> MASWSHPQFEKGSTSAFNPRDTVTVYFHAIVSRHFGFNPEEHKVYVRGGEGLGQKGWTDACEMYCTQDLHDLGSLVEGKMDIPRQSLDKPIPYKYVIHRGGSSKDTVEYEFIYEQAQKKGEHVNRCLRVVSTSLGNGDWHQYDDIICMRSTGFFQQAKNRILDSTRKELLKGKKQAAVVMLDRIFSVLQPWSDINLQSFMTQFLQFYSVVREPMIHDGRARKWTSLQYEEKEVWTNLWEHVKKQMAPFLEGKSGESLPADCPVRSKLTLGLSILFMVEAAEFTVPKKDLDSLCYLLIPSAGSPEALHSDLSPVLRIRQRWRIYLTNLCLRCIDERCDRWLGILPLLHTCMQKSPPKKNSKSQPEDTWAGLEGISFSEFRDKAPTRSQPLQFMQSKMALLRVDEYLFRSWLSVVPLESLSSYLENSIDYLSDVPVRVLDCLQGISYRLPGLRKISNQNMKKDVENVFKMLMHLVDIYQHRIFGENLLQIYLTECLTLHETVCNITANHQFFEIPALSAELICKLLELSPPGHTDEGLPEKSYEDLVTSTLQEALATTRNWLRSLFKSRMLSISSAYVRLTYSEEMAVWRRLVEIGFPEKHGWKGSLLGDMEGRLKQEPPRLQISFFCSSQCRDGGLHDSVSRSFEKCVIEAVSSACQSQTSVLEGLSCQDLQKFGTLLSAVITKSWPVHNGEPVFDVDEIFKYLLKWPDVRQLFELCGTNEKIIDNITEEGRQLMATAESVFQKVAGELENGTIVVGQLELILEHQSQFLDIWNLNRRRLPSQEKACDVRSLLKRRRDDLLFLKQEKRYVESLLRQLGRVKHLVQVDFGNIEIIHSQDLSNKKLNEAVIKLPNSSSYKRETHYCLSPDIREMASKLDSLKDSHIFQDFWQETAESLNTLDKDPRELKVSLPEVLEYLYNPCYDNFYTLYENLKSGKITFAEVDAIFKDFVDKYDELKNDLKFMCTMNPQDQKGWISERVGQIKEYHTLHQAVSSAKVILQVRRALGVTGDFSVLNPLLNFADSFEDFGNEKLDQISPQFIKAKQLLQDISEPRQRCLEELARQTELVAWLHKALEDINELKVFVDLASISAGENDIDVDRVACFHDAVQGYASLLYKMDERTNFSDFMNHLQELWRALDNDQHLPDKLKDSARNLEWLKTVKESHGSVELSSLSLATAINSRGVYVIEAPKDGQKISPDTVLRLLLPDGHGYPEALRTYSTEELKELLNKLMLMSGKKDHNSNTEVEKFSEVFSNMQRLVHVFIKLHCAGNMLFRTWTAKVYCCPDGGIFMNFGLELLSQLTEKGDVIQLLGALCRQMEDFLDNWKTVVAQKRAEHFYLNFYTAEQLVYLSSELRKPRPSEAALMMLSFIKGKCTVQDLVQATSACESKADRYCLREVMKKLPQQLLSEPSLMGKLQVIMMQSLVYMSAFLPHCLDLDALGRCLAHLATMGGTPVERPLPKGLQAGQPNLILCGHSEVLPAALAIYMQAPRQPLPTFDEVLLCTPATTIEEVELLLRRCLTSGSQGHKVYSLLFADQLSYEVGCQAEEFFQSLCTRAHREDYQLVILCDAAREHCYIPSTFSQYKVPLVPQAPLPNIQAYLQSHYQVPKRLLSAATVFRDGLCVGIVTSERAGVGKSLYVNTLHTKLKAKLRDETVPLKIIRLTEPHLDENQVLSALLPFLKEKYQKMPVIFHIDISTSVQTGIPIFLFKLLILQYLMDINGKIWRRSPGHLYLVEIPQGLSVQPKRSSKLNARAPLFKFLDLFPKVTCRPPKEVIDMELTPERSHTDPAMDPVEFCSEAFQRPYQYLKRFHQQQNLDTFQYEKGSVEGSPEECLQHFLIYCGLINPSWSELRNFAWFLNCQLKDCEASIFCKSAFTGDTLRGFKNFVVTFMILMARDFATPTLHTSDQSPGRQSVTIGEVVEEDLAPFSLRKRWESEPHPYVFFNGDHMTMTFIGFHLETNNNGYVDAINPSNGKVIKKDVMTKELFDGLRLQRVPFNIDFDNLPRYEKLERLCLALGIEWPIDPDETYELTTDNMLKILAIEMRFRCGIPVIIMGETGCGKTRLIKFLSDLKRGSVEAETMKLVKVHGGTTPSMIYSKVKEAERTAFSNKAQHKLDTILFFDEANTTEAVSCIKEILCDRTVDGEHLHEDSGLHIIAACNPYRKHSQEMILRLESAGLGYRVSAEETADRLGSIPLRQLVYRVHALPPSLIPLVWDFGQLNDSAEKLYIQQIVQRLVDSVSVNPSETCVIADVLSASQMFMRKRENECGFVSLRDVERCVKVFRWFHDHSDMLLKELDKFLHESSDSTHTFERDPVLWSLVMAIGVCYHASLEEKASYRTAIARCFPKPYNSSRAILDEVTHVQDLFLRGAPIRTNIARNLALKENVFMMVICIELKIPLFLVGKPGSSKSLAKIIVADAMQGQAAFSELFRCLKQVHLVSFQCSPHSTPQGIISTFKQCARFQQGKDLGQYVSVVVLDEVGLAEDSPKMPLKTLHPLLEDGCIEDDPAPYKKVGFVGISNWALDPAKMNRGIFVSRGSPNEKELIESAEGICSSDRLVQDKIRGYFAPFAKAYETVCQKQDKEFFGLRDYYSLIKMVFAKAKASKRGLSPQDITHAVLRNFSGKDNIQALSIFTASLPEARYKEEVSTVELIKQNIYPGPQASSRGLDGAESRYLLVLTRNYVALQILQQTFFEGQQPEIIFGSSFPQDQEYTQICRNINRVKICMETGKMVVLLNLQNLYESLYDALNQYYVYLGGQKYVDLGLGTHRVKCRVHTAFRLIVIEEKDVVYKQFPVPLINRLEKHYLDMNTVLQPWQKSIVQELQQWAHEFADVKADQFIARHKYSPADVFIGYHSDACASVVLQAVERQGCRDLTEELYRKVSEEARSILLDCATPDAVVRLSGSSLGSFTAKQLSQEYYYAQQHNSFVDFLQAHLRMTHHECRAVFTEITTFSRLLTGNDCDVLASELRGLASKPVVLSLQQYDTEYSFLKDVRSWLTNPGKRKVLVIQADFDDGTRSAQLVASAKYTAINEINKTQGTKDFVFVYFVTKLSRMGSGTSYVGFHGGLWRSVHIDDLRRSTIMASDVTKLQNVTISQLFKPEDKPEQEEMEIETSQSKELAEEQMEVEDSEEMKKASDPRSCDCSQFLDTTRLVQSCVQGAVGMLRDQNESCARNMRRVTILLDLLNEDNTRNASFLRESKMRLHVLLNKQEENQVRSLKEWVTREAANQDALQEAGTFRHTLWKRVQDVVTPILASMIAHIDRDGNLELLAQPDSPAWVQDLWMFIYSDIKFLNISLVLNNTRSNSEMSFILVQSHMNLLKDAYNAVPFSWRIRDYLEELWVQAQYITDTEGLSKKFVEIFQKTPLGVFLAQFPVAQQQKLLQSYLKDFLLLTMKVSSREELMFLQMALWSCLRELQEASGTPDETYKFPLSLPWVHLAFQHFRTRLQNFSRILTIHPQVLSSLSQAAEKHSLAGCEMTLDAFAAMACAEMLKGDLLKPSPKAWLQLVKNLSTPLELVCSEGYLCDSGSMTRSVIQEVRALWNRIFSIALFVEHVLLGTESHIPELSPLVTTYVSLLDKCLEEDSNLKTCRPFVAVMTTLCDCKDKASKKFSRFGIQPCFICHGDAQDPVCLPCDHVYCLRCIQTWLIPGQMMCPYCLTDLPDKFSPTVSQDHRKAIEKHAQFRHMCNSFFVDLVSTMCFKDNTPPEKSVIDTLLSLLFVQKELLRDASQKHREHTKSLSPFDDVVDQTPVIRSVLLKLLLKYSFHEVKDYIQNYLTQLEKKAFLTEDKTELYLLFISCLEDSVHQKTSAGCRNLEQVLREEGHFLRTYSPGLQGQEPVRIASVEYLQEVARVRLCLDLAADFLSELQEGSELAEDKRRFLKHVEEFCTRVNNDWHRVYLVRKLSSQRGMEFVQSFSKQGHPCQWVFPRKVIAQQKDHVSLMDRYLVHGNEYKAVRDATAKAVLECKTLDIGNALMACRSPKPQQTAYLLLALYTEVAALYRSPNGSLHPEAKQLEAVNKFIKESKILSDPNIRCFARSLVDNTLPLLKIRSANSILKGTVTEMAVHVATILLCGHNQILKPLRNLAFYPVNMANAFLPTMPEDLLVHARTWRGLENVTWYTCPRGHPCSVGECGRPMQESTCLDCGLPVGGLNHTPHEGFSAIRNNEDRTQTGHVLGSPQSSGVAEVSDRGQSPVVFILTRLLTHLAMLVGATHNPQALTVIIKPWVQDPQGFLQQHIQRDLEQLTKMLGRSADETIHVVHLILSSLLRVQSHGVLNFNAELSTKGCRNNWEKHFETLLLRELKHLDKNLPAINALISQDERISSNPVTKIIYGDPATFLPHLPQKSIIHCSKIWSCRRKITVEYLQHIVEQKNGKETVPVLWHFLQKEAELRLVKFLPEILALQRDLVKQFQNVSRVEYSSIRGFIHSHSSDGLRKLLHDRITIFLSTWNALRRSLETNGEIKLPKDYCCSDLDLDAEFEVILPRRQGLGLCGTALVSYLISLHNNMVYTVQKFSNEDNSYSVDISEVADLHVISYEVERDLNPLILSNCQYQVQQGGETSQEFDLEKIQRQISSRFLQGKPRLTLKGIPTLVYRRDWNYEHLFMDIKNKMAQSSLPNLAISTISGQLQSYSDACEALSIIEITLGFLSTAGGDPGMDLNVYIEEVLRMCDQTAQVLKAFSRCQLRHIIALWQFLSAHKSEQRLRLNKELFREIDVQYKEELSTQHQRLLGTFLNEAGLDAFLLELHEMIVLKLKGPRAANSFNPNWSLKDTLVSYMETKDSDILSEVESQFPEEILMSSCISVWKIAATRKWDRQSRGGGHHHHHHHHHH;> GWSHPQFEKPGSMAASRRLMKELEEIRKSGMKNFRNIQVDEANLLTWQGLIVPDNPPYDKGAFRIEINFPAEYPFKPPKITFKTKIYHPNIDEKGQVCLPVISAENWKPATKTDQVIQSLIALVNDPQPEHPLRADLAEEYSKDRKKFSKNAEEFTKKYGEKRPVD

The giant E3 ubiquitin ligase RNF213 is a conserved component of mammalian cell-autonomous immunity, limiting the replication of bacteria, viruses and parasites. RNF213 is the largest E3 Ub ligase (E3) in the human proteome, combining E3 and AAA (ATPases Associated with diverse Activities) modules into a single ~600 kDa polypeptide. The cryo-EM structure of M. musculus RNF21328 revealed that RNF213 comprises three sub-modules: an N-terminal stalk, a dynein-like AAA core consisting of six ATPase units (only the two units AAA3 and AAA4 can bind and hydrolyze ATP), and a composite E3 module, including a RING domain. Thus, ATP binding to AAA3 and AAA4 subunits is necessary and sufficient to promote the E3 ligase activity of RNF213.

As prior data (RING domain independence and activity with UBE2L328) suggested RNF213 could be a transthiolating E3 (i.e. covalently receives Ub from E2~Ub onto an active site cysteine), we used an activity-based probe (ABP) based on an E2~Ub conjugate, specific for this class of E3 mechanism. The probe structurally mimics E2~Ub but is chemically modified to undergo irreversible covalent labeling of an E3’s active site cysteine during transthiolation. Based on previous biochemical and proteomics data, we used the E2 UBE2L3 to generate the ABP and appended a biotin tag to enable detection (biotin-ABP). The 3.5 Å structure, revealed that UBE2L3 is bound via a well-defined interface formed between the C-terminal domain (CTD) of RNF213 and the L1/L2 loops and H1 helix of UBE2L3. CTD residues Phe5093, Trp5097, and Tyr5106 are oriented to undergo hydrophobic interactions with Phe63 and Pro97 located on the UBE2L3 L1 and L2 loops, respectively. This contact is putatively strengthened by nearby electrostatic interactions formed between CTD Glu5108 and Arg6 in the UBE2L3 H1 helix, and CTD Asp5101 and Lys96 in the UBE2L3 L2 loop. As nucleotides were absent from sites AAA3 and AAA4 in our RNF213-E2-Ub structure, we postulated that RNF213 might have reverted to an inactive conformation during sample processing, rendering our structure a covalently linked “footprint” of the activated transthiolation intermediate. To explore this possibility, we generated a second cryo-EM structure where the ATPγS-stimulated ABP labeling reaction was applied directly to cryo-EM grids. Modest structural changes were evident (RMSD = 2.66 Å) in the AAA core and new density at the AAA3 and AAA4 sites allowed modeling of ADP. However, there remained no clear density for the RZ domain nor Ub and no apparent basis for activation of transthiolation.> GWARGAPRPPPSSPPLSIMGLMPLTKEVAKGSIGRGVLPAVELAIEQIRNESLLRPYFLDLRLYDTECDNAKGLKAFYDAIKYGPNHLMVFGGVCPSVTSIIAESLQGWNLVQLSFAATTPVLADKKKYPYFFRTVPSDNAVNPAILKLLKHYQWKRVGTLTQDVQRFSEVRNDLTGVLYGEDIEISDTESFSNDPCTSVKKLKGNDVRIILGQFDQNMAAKVFCCAYEENMYGSKYQWIIPGWYEPSWWEQVHTEANSSRCLRKNLLAAMEGYIGVDFEPLSSKQIKTISGKTPQQYEREYNNKRSGVGPSKFHGYAYDGIWVIAKTLQRAMETLHASSRHQRIQDFNYTDHTLGRIILNAMNETNFFGVTGQVVFRNGERMGTIKFTQFQDSREVKVGEYNAVADTLEIINDTIRFQGSEPPKDKTIILEQLRKISLPLYSILSALTILGMIMASAFLFFNIKNRNQKLIKMSSPYMNNLIILGGMLSYASIFLFGLDGSFVSEKTFETLCTVRTWILTVGYTTAFGAMFAKTWRVHAIFKNVKMKKKIIKDQKLLVIVGGMLLIDLCILICWQAVDPLRRTVEKYSMEPDPAGRDISIRPLLEHCENTHMTIWLGIVYAYKGLLMLFGCFLAWETRNVSIPALNDSKYIGMSVYNVGIMCIIGAAVSFLTRDQPNVQFCIVALVIIFCSTITLCLVFVPKLITLRTNPDAATQNRRFQFTQNQKKEDSKTSTSVTSVNQAS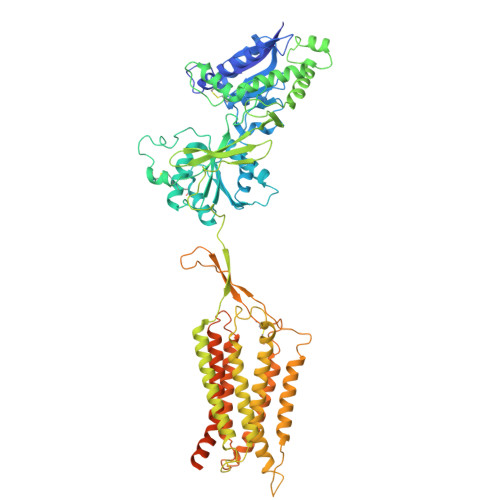TSRLEGLQSENHRLRMKITELDKDLEEVTMQLQDT> MAVPIAQKSEPHSLSSEALMRRAVSLVTDSTSTFLSQTTYALIEAITEYTKAVYTLTSLYRQYTSLLGKMNSEEEDEVWQVIIGARAEMTSKHQEYLKLETTWMTAVGLSEMAAEAAYQ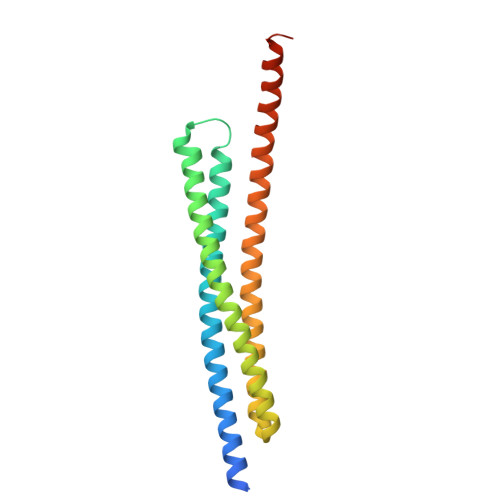TGADQASITARNHIQLVKLQVEEVHQLSRKAETKLAEAQIEELRQKTQEEGEERAESEQEAYLREDHHHHHHHHH>MYTNSDFVVIKALEDGVNVIGLTRGADTRFHHSEKLDKGEVLIAQFTEHTSAIKVRGKAYIQTRHGVIESEGKK[22x]

Specific damage manifestations were determined within the large trp RNA-binding attenuation protein (TRAP) bound to a single-stranded RNA that forms a belt around the protein. TRAP consists of 11 identical subunits assembled into a ring with 11-fold rotational symmetry. For crystalline complexes such as C.Esp1396I, whether the protein is intrinsically more susceptible to X-ray-induced damage or whether the protein scavenges electrons to protect the DNA remains unclear in the absence of a non-nucleic acid-bound protein control obtained under exactly the same crystallization and data-collection conditions. To monitor the effects of nucleic acid binding on protein damage susceptibility, a crystal containing two protein molecules per asymmetric unit, only one of which was bound to RNA, is reported here. In this structure, the bases of the G1-A2-G3 nucleotides form direct hydrogen bonds to the protein, unlike the U4-U5 nucleotides, which appear to be more flexible.

Here, a methodology has been developed whereby per-atom density changes could be quantified with increasing dose over a wide (1.3–25.0 MGy) range and at higher resolution (1.98 Å) than the previous systematic specific damage study on a protein–DNA complex. Over a large dose range, the RNA was found to be far less susceptible to radiation-induced chemical changes than the protein. The 11-fold symmetry within each TRAP ring permitted statistically significant analysis of the Glu and Asp damage patterns, with RNA binding unexpectedly being observed to protect these otherwise highly sensitive residues within the 11 RNA-binding pockets distributed around the outside of the protein molecule. Additionally, the method enabled a quantification of the reduction in radiation-induced Lys and Phe disordering upon RNA binding directly from the electron density. RNA interacting with TRAP was shown to offer significant protection against radiation-induced structural changes.> GPLGSMSSLSASAENVSSLGLGSGGGGTNSHDGNSQQGSGSDGGSSMCLELALEGERLCNAGDCRAGVAFFQAAIQAGTEDLRTLSAIYSQLGNAYFYLGDYNKAMQYHKHDLTLAKSMNDRLGEAKSSGNLGNTLKVMGRFDEAAICCERHLTLARQLGDRLSEGRALYNLGNVYHAKGKHLGQRNPGKFGDDVKEALTRAVEFYQENLKLMRDLGDRGAQGRACGNLGNTYYLLGDFQAAIEHHQERLRIAREFGDRAAERRANSNLGNSHIFLGQFEDAAEHYKRTLALAVELGEREVEAQSCYSLGNTYTLLHEFNTAIEYHNRHLAIAQELGDRIGEARACWSLGNAHSAIGGHERALKYAEQ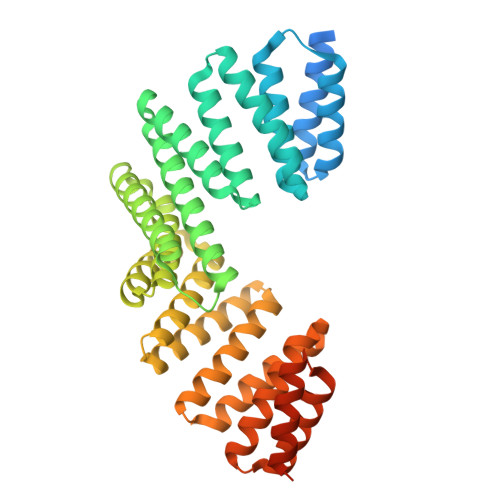HLQLAXXXXXXXXXXXXXXXXXXXXXXXXXXXXXXXXXXXXXX>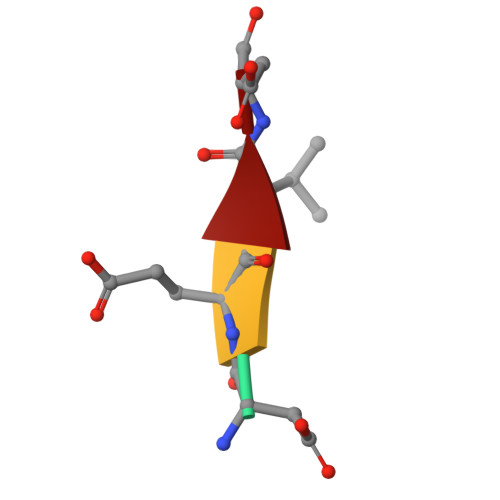 DEVD> IVGGQECKDGECPWQALLINEENEGFCGGTIL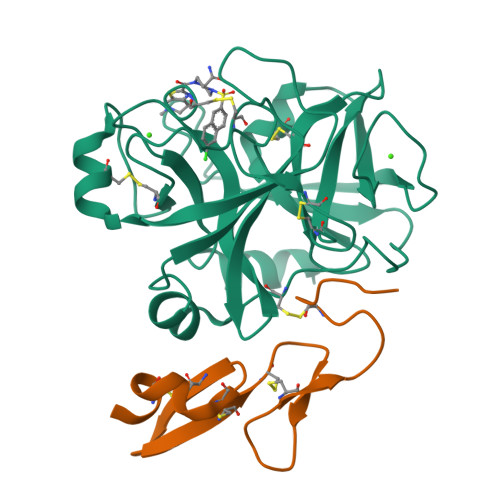SEFYILTAAHCLYQAKRFKVRVGDRNTEQEEGGEAVHEVEVVIKHNRFTKETYDFDIAVLRLKTPITFRMNVAPACLPERDWAESTLMTQKTGIVSGFGRTHEKGRQSTRLKMLEVPYVDRNSCKLSSSFIITQNMFCAGYDTKQEDACQGDSGGPHVTRFKDTYFVTGIVSWGEGCARKGKYGIYTKVTAFLKWIDRSMK;> KLCSLDNGDCDQFCHEEQNSVVCSCARGYTLADNGKACIPTGPYPCGKQTLE>[4x]MARIIENNVGGVALTFDDVLLRPEFSNVLPRDIDISTRIAKDFTLNLPIMSAAMDQVTDSRLAIAMAQAGGLGVIHRNFSPSEQVAQVHQVKKFESGGVKDIERSQLNPNATKDSKGRLRVAAAVSVAKDIADRVGPLFDVNVDLVVVDTAHGHSQKVLDAVVQIKKNFPSLLVMAGNIATAEGALALIDAGADIIKVGIGPGSICTTRVV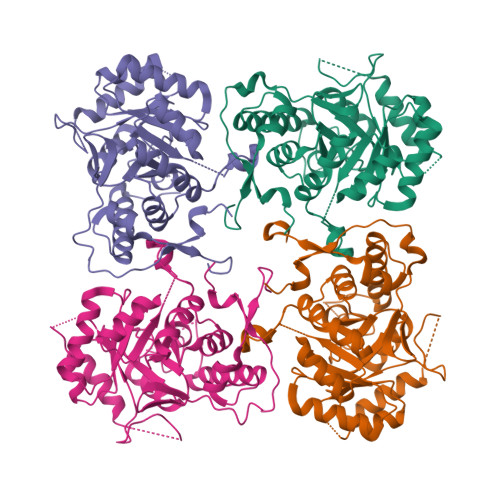TGVGCPQLSAIMSVVEVAERAGVAIVADGGIRFSGDIAKAIAAGSACVMIGSLLAGTDESPGDIFLYQGRSFKSYRGMGSVAAMERGSSARYSQDGVTDVLKLVPEGIEGRVPYKGPIASVLHQMSGGLKSSMGYVGASNIEEFQKKANFIRVSVAGLRESHVHDVKITRESPNYSETI> KLFEHT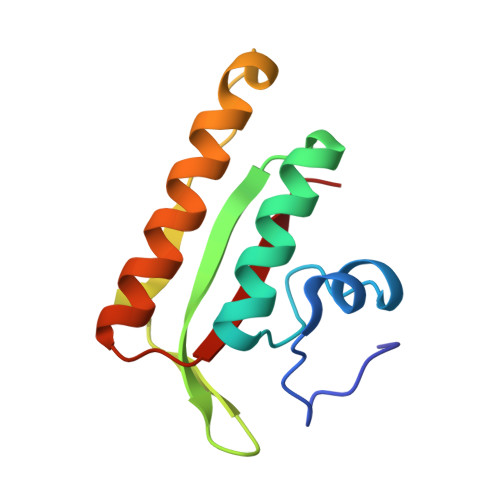VLYDSGDAFFELKGNASMKLSPKAAIEVCNEAAKKGLWILGIDGGHWLNPGFRIDSSASWTYDMPEEYKSKIPENNRLAIENIKDDIENGYTAFIITLKM>MGTAQSVILPLPSDHARFISLRLKDLSVAELKKHIALLHSTRDRLITQHPAAQIKAAVAFGPEIWLQLYKEMPSGFKQLAPQQGTFQMPVVPADVFIHIASARADICFALSQAFFEGIKDKVEVLDERVCFRYFDGRDITGFIDGTENPQFNDDRAEVALLPEDSGVFADGSFIFAQRYAHDLEKWKRLKVDTQEQIMGRTKLESIELDNEVKPENAHIARTVVEDENGEEMEILRHSLPYGDGKGDQGLFFIAYTKDL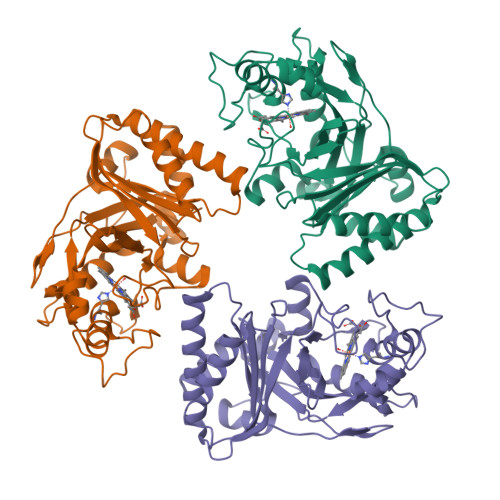NIIDLMLNRMFGTSGDGIHDRLLHFVTPLDGAYYFAPSAELLEVILESLEHHHHHH[3x]>MSNCQYKIYPPLGIARVGNGPAIKPLSLSTPEVPWAHLYDTNVQYLVTQQELEQLLEEAFGGNVINEISQIKTKLDERKAEKFKQEEIETITGLLGLSHLVPQQQLSRSLDNLELKSTKDSDDIVQQIKGALLKVLSDHYLHAVKKQAQNFYIYKCDEQGNPVEKLKLTDGDKVTWRVEVANKKSFWYDYNNALDLSLHTQGSGNLSKNVSKHRLAPAMTAKRRNPNVITNSLRKQLVISSQGSVSSDNNTQVPLRGKFPANEPDTNNRLSDLLNLQERHNVLQGSIECDNEGVLRFYAGNGISQALSPSSLNTDFADNSNWFDDICDGRVTAVVELKNGDTFEIQDEQSSAWVATTPPDYAP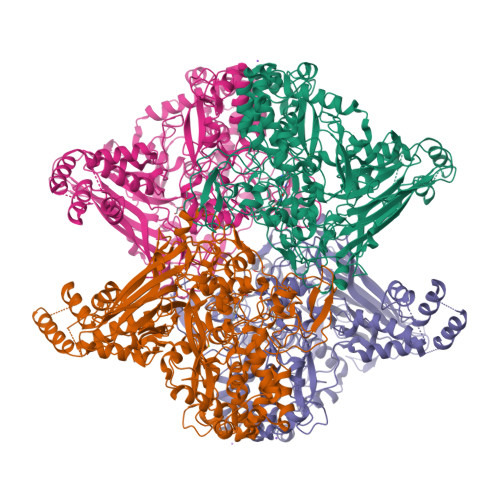QIEPIVTMYDMVSGAALKEQDLDNLTTQFSDVFPILYRLYRMQWVNQADFTDNAVNTQIRELNSELGFAQLLDNSASAKSLREGIFNQFRNPLFDQDIDVDDPGQSSNEWVSNSRIIPSKDETNIAAKPATSSLKLPFYPNDGIDYPGSPVQWFAIPPFMYQHLQNWAAGDFSVTQVEKESANTIEELGLFYSEQFKNSPNSALLCARGALDALYGGGFHPGVELTWPMRHNLIYSQNDYVSSVTPEINLLGLREFRLKQDLQGLNSPNMYQDFGHVIAVDNVTASIDPNSDAAWLWRSTPGDLTKWMGIPWQSDAASCQAVYTPEDFPIPSWXAANLPVHVLPLARYNKFKDSQSADLPEINGMTHSIAQGMSEETFEHLRLEQFSQRLDWLHTADLGFVGYHAEGGYTNGLIQMVSQWKNMAMVMARPVENPGSSGIPNVVYVAYSQADKD[4x]(2S)-3-(4-chloro-3-fluorophenoxy)-N-[4-cyano-3-(trifluoromethyl)phenyl]-2-hydroxy-2-methylpropanamide 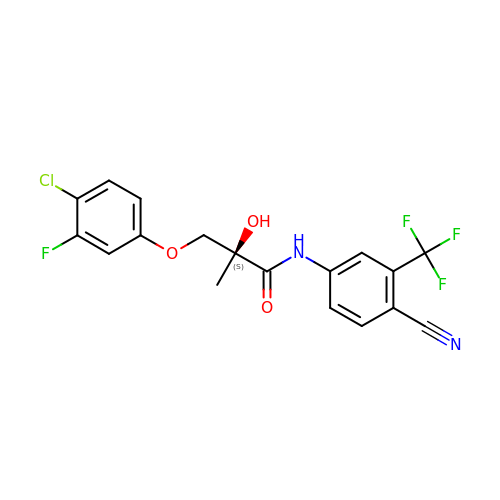| C18 H13 Cl F4 N2 O3 | SSFVOEAXHZGTRJ-KRWDZBQOSA-N4-[(1-{(1S,2S)-1-[1-(4-aminobutyl)-1H-1,2,3-triazol-4-yl]-2-methylbutyl}-1H-1,2,3-triazol-4-yl)methoxy]-3-methoxybenzene-1-carboximidamide 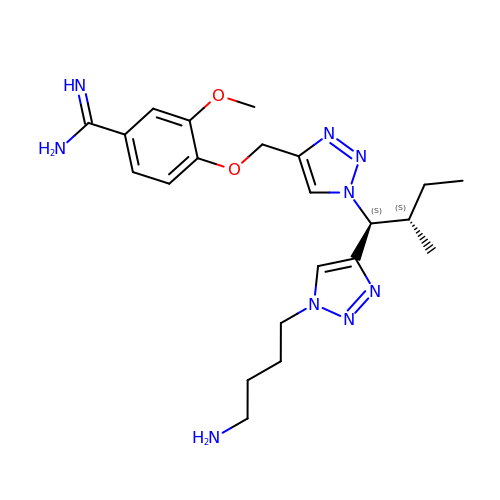| C22 H33 N9 O2 | DNIWQYWTKVVYDZ-BTYIYWSLSA-N>[2x]SDCD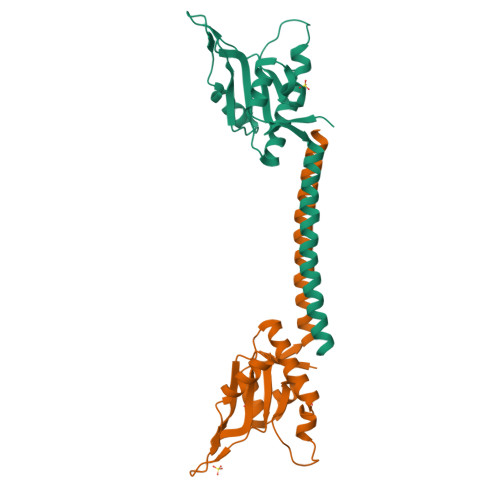HDEKLVYPWKGIVVNIPTTKAQDGRSAGESGSKLRDEYILRGFNPTRVRPLWNYLGHSGTAIVEFNKDWNGLHNGLLFDKAYTVDGHGKKDWLKKDGPKLGLYGWIARADDYNGNNIIGENLRKTGDLKTIAELTEEEARKQELLVQNLRQLVEEKKKDMKEIEELCS>MQAGPAMERHYYTYLIKEEFANHYFGRESVMFELFQDYHWTSLEKQQYEMTEKQIQYITQPIPILHMHQRLKMNLNKTDYRQLDYIYRIALPKAKGHATFMMKEHMIEIVASGDYEAETIFFEVLRKVSPCFLAMDFNSKRYGWLNPVKERNFV[2x];>GPAMENILDLWNQALAQIEKKLSKPSFETWMKSTKAHSLQGDTLTITAPNEFARDWL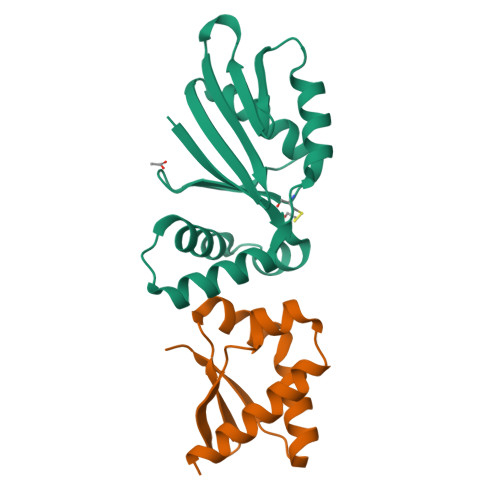ESRYLHLIADTIYELTGEELSIKFVIPQ[2x]>[3x]GHMASIINITELNISGCYLIESPIFSDERGEFVKTHHQEIFKNFGLEIPSAEEYYSRSKNNVIRGMHFQQYPDDHNKLVFCPEGEVLDVFLDIRKDSNTYGQF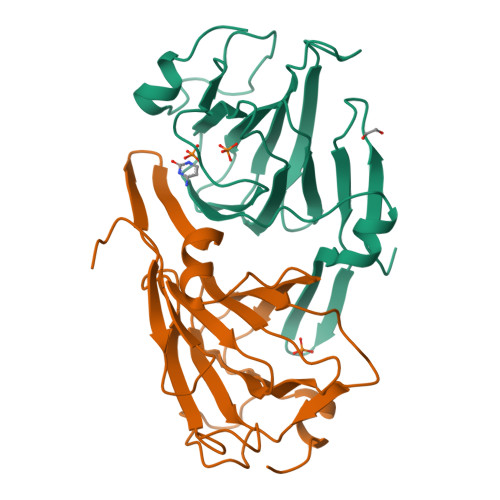MSFILNPHNRRSIFLAKGIAHGFLSMKDNTLIVCKTSTVHSPSRDSGIHWNSFGFKWPVENPIISDKDRNLDCFF~{N}-[(2~{R},3~{R},4~{R},5~{S},6~{R})-6-(hydroxymethyl)-5-[(2~{S},3~{R},4~{S},5~{S},6~{R})-6-(hydroxymethyl)-3,5-bis(oxidanyl)-4-(1~{H}-1,2,3-triazol-4-ylmethoxy)oxan-2-yl]oxy-4-oxidanyl-2-propoxy-oxan-3-yl]ethanamide | C20 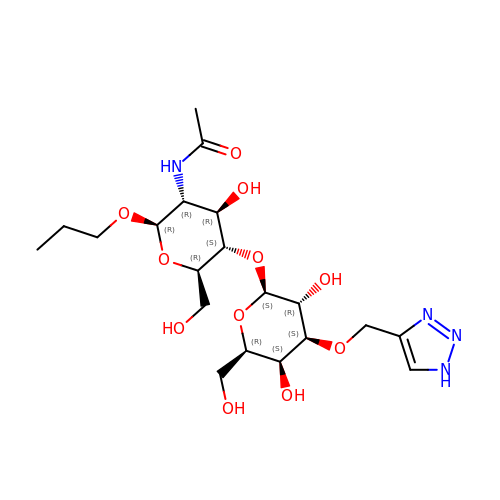H34 N4 O11 | BHUHIMJWCDUIMU-MRHFAZSRSA-N> GAMGSFNSSINNIHEMEIQLKDALEKNQ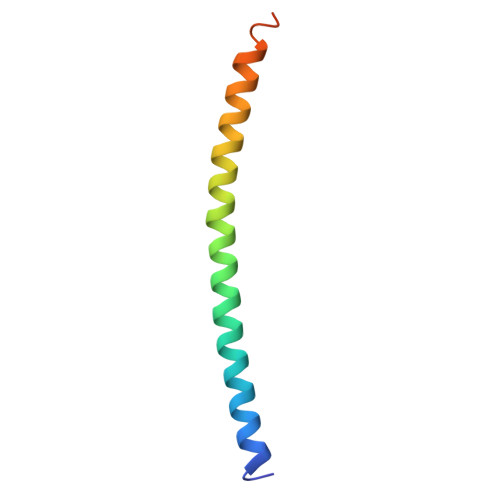QWLVYDQQREVYVKGLLAKIFELEKKTETAAHSLP>[2x]GLVPRGSHMAYISLNYHSPTIGMHQNLTVILPEDQSFFNSDTTVKPLKTLMLLHGLSSDETTYMRYTSIERYANEHKLAVIMPNVDHSAYANMAYGHSYYDYILEVYDYVHQIFPLSKKRDDNFIAGHSMGGYGTIKFALTQGDKFAKAVPLSAVFEAQNLMDLEWNDFSKEAIIGNLSSVKGTEHDPYYLLDKAVAEDKQIPKLLIMCGKQDFLYQDNLDFIDYLSRINVPYQFEDGPGDHDYAYWDQAIKRAITWMVND

Here we identify the bacterial esterases, GloB and FrmB, that activate carboxy ester prodrugs in Staphylococcus aureus. To establish the structural basis for FrmB and GloB substrate specificity and enable future structure-guided prodrug therapeutic design, we solved the three-dimensional structures of both S. aureus FrmB and GloB. FrmB and GloB have distinct ester substrate specificities, which are supported by the structures of their active sites. Additionally, the finding that mutation in either frmB or gloB is sufficient to confer POM-HEX resistance suggests that the two enzymes may work in concert to bioconvert POM-HEX into HEX.

Conversely, FrmB orthologs hydrolyze p-nitrophenyl esters of short-chain fatty acids (C2–C6) and are thought to mediate detoxification of cellular formaldehyde. A single dimer of FrmB is observable in the asymmetric unit, matching the apparent molecular weight of FrmB as observed via size-exclusion chromatography. The overall fold of FrmB is characteristic of the α/β-hydrolase fold. Six parallel β-strands and one anti-parallel β-strand pair form a central eight stranded β-sheet, which is surrounded by α-helices. One monomer of FrmB has electron density for a single magnesium ion, whereas the second monomer has two magnesium ions present. All structures display strong structural conservation including the positioning of the prototypic serine hydrolase catalytic triad: Ser120, Asp204, and His233 (S. aureus). However, SaFrmB and human esterase D differ notably in the solvent-accessible surface around the active site, suggesting the potential for distinct substrate utilization, primarily driven by differential positioning of the cap domain. Using Autodock Vina, we modeled the highest catalytic efficiency substrate of FrmB, 1O, onto the active site of FrmB. The pocket directly next to the oxyanion hole is relatively narrow, suggesting that steric hindrance explains the poor activity of FrmB against branched substrates. The active site pocket extends and opens significantly after passing by the oxyanion hole, supporting the capacity of FrmB to hydrolyze substrates that contain large steric groups distant from the carbonyl carbon, such as 11O.> MAIYADNSYSIGNTPLVRLKHFGHNGNVVVKIEGRNPSYSVKCRIGANMVWQAEKDGTLTKGKEIVDATSGNTGIALAYVAAARGYKITLTMPETMSLERKRLLCGLGVNLVLTEGAKGMKGAIAKAEEIVASDPSRYVMLKQFENPANPQIHRETTGPEIWKDTDGKVDVVVAGVGTGGSITGISRAIKLDFGKQITSVAVEPVESPVISQTLAGEEVKPGPHKIQGIGAGFIPKNLDLSIIDRVETVDSDTALATARRLMAEEGILAGISSGAAVAAADRLAKLPEFAD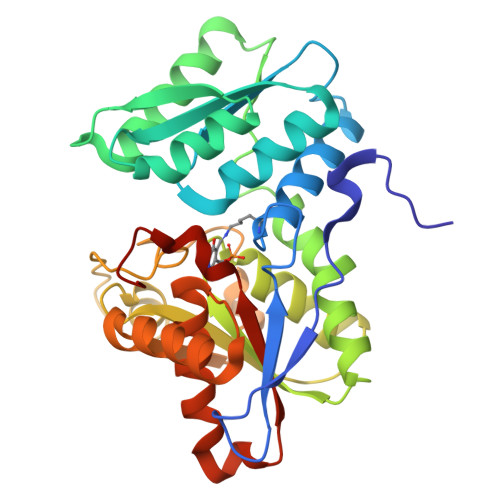KLIVVILPSASERYLSTALFEGIEG>[18x]GAVVRST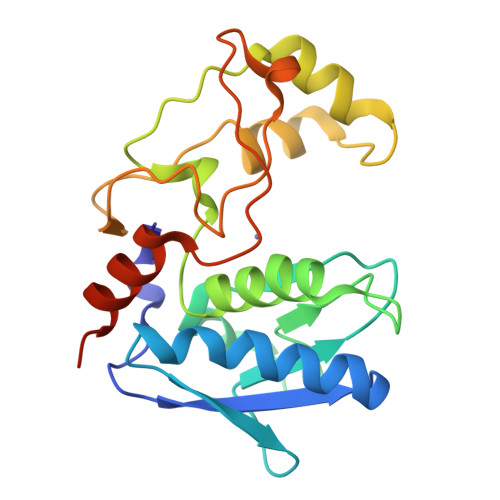KWPNGSVITVGLYGGTPYVRSKVKQYAQEWSNYANITFNFVESGTPQIRVTFTQGAGSYSYLGTQALSIPSNEETMNFGWFDDSTSDTEFSRTVIHEFGHALGMIHEHQHPLTNIPWDKNKVYAYYAGYPNYWSKKDVDNNLFATYSTTQTQYSAYDTQSIMHYSISSALTTNGFSVGNNSVLSATDKQFIATVYPRNLEHHHHHH DNMT2 (TRDMT1) is a human RNA methyltransferase implicated in various disease processes. Instead of DNA, which is the main target of DNMT1 and DNMT3, DNMT2 introduces the m5C38 modification in several tRNAs. Physiologically, DNMT2 targets various tRNAs, including tRNAGly, tRNAVal, and tRNAAsp.9,12 tRNA methylation by DNMT2 plays a role in regulating RNA degradation by ribonucleases, thereby enhancing tRNA stability and overall protein expression. Additionally, tRNA m5C38 methylation improves codon recognition, particularly distinguishing between aspartate and glutamate, thus enhancing translational accuracy.

For our crystallographic studies, we used a deletion construct of human DNMT2, dubbed DNMT2Δ47, in which residues 191 to 237 were deleted since this region is predicted as intrinsically disordered. The asymmetric unit contains two very similar DNMT2Δ47-compound 3 complexes with an overall rmsd(Cα) of 0.354 Å and the largest differences in the loop region comprising residues 82 to 95. We could show that DNMT2Δ47 with bound compound 3 is indeed dimeric in solution at a high protein concentration of 10 mg/mL, which was also used for crystallization. Most interestingly, compound 3 is bound in a largely hydrophobic pocket adjacent to the active site. The indole ring of compound 3 is located in a hydrophobic cave formed by Y10, M75, backbone of S76, P77, F99, L118, F124, and L133. Additionally, the amine group of the indole ring forms a hydrogen bond with the backbone carbonyl of E119. The amide group, which connects the ethylbenzene and cyclopropane moieties, is in van der Waals contact with P78 and R95 and forms three hydrogen bonds, namely with the main chain carbonyl of L278B, with the side chain of N120, and an intramolecular H-bond to the amino group connecting the cyclopropane and indole moieties. The largest local movement upon binding of compound 3 is observed in the loop following β4 (M75 to P78), where P77 and P78 are rotated and shifted toward the SAH binding site. Moreover, the active site residue C79 is now resolved and moved into the SAH binding region. The superposition depicted in Figure 4D shows that binding of compound 3 narrows the active site, which prohibits SAH binding due to steric hindrance by P77, P78, and C79. As a consequence, compound 3 acts as an allosteric inhibitor by reshaping the active site.

>GAMEPLRVLELYSGVGGMHHALRESCIPAQVVAAIDVNTVANEVYKYNFPHTQLLAKTIEGITLEEFDRLSFDMILMSPPCQPFTRIGRQGDMTDSRTNSFLHILDILPRLQKLPKYILLENVKGFEVSSTRDLLIQTIENCGFQYQEFLLSPTSLGIPNSRLRYFLIAKLQSEPLPFQAPGQVLMEFPKIESEIHRKNQQDSDLSVKMLKDFLEDDTDVNQYLLPPKSLLRYALLLDIVQPTCRRSVCFTKGYGSYIEGTGSVLQTAEDVQVENIYKSLTNLSQEEQITKLLILKLRYFTPKEIANLLGFPPEFGFPEKITVKQRYRLLGNSLNVHVVAKLIKILYE[2x]ORF8 is a viral immunoglobulin-like (Ig-like) domain protein encoded by the severe acute respiratory syndrome coronavirus 2 (SARS-CoV-2) RNA genome. It tends to evolve rapidly and interfere with immune responses. The full-length SARS-CoV-2 ORF8 is composed of a signal peptide (residues 1-15) and an Ig-like domain (residues 16-121). Herein, we determined the crystal structures of SARS-CoV-2 ORF8 (S84) (one of the epidemic isoforms) and the bat coronavirus RaTG13 ORF8 variant at 1.62 Å and 1.76 Å resolution, respectively.

To determine the sequence-structure relationship, we next solved the crystal structure of the RaTG13 ORF8 Ig-like domain at 1.76 Å, in which the electron density of residues 18-121 can be clearly traced. It is worth noting that there are two molecules in one asymmetric unit, which is different from SARS-CoV-2 ORF8 (S84). Protomers A and B form a dimer via an intermolecular covalent Cys20-Cys20 disulfide bond. Similar to SARS-CoV-2 ORF8, the RaTG13 ORF8 Ig-like domain folds into a “β-sandwich” containing two β-sheets (strands βB, βD, and βE compose the small sheet; strands βA, βC, βC’, βF, and βG compose the large sheet) and an insertion region. However, the insertion region forms a dynamic loop in the RaTG13 ORF8 Ig-like domain, distinguished from the β-hairpin fold in SARS-CoV-2 ORF8 (S84). Unlike SARS-CoV-2 ORF8 (S84), the residues 62-78 loop region of RaTG13 ORF8 is assembled different conformations between the protomer A and protomer B in one asymmetric unit. The electron density of residues 63-65 of RaTG13 ORF8 is unclear, indicating a dynamic region. Additionally, the RaTG13 ORF8 displayed a similar two-stranded parallel β-sheet in protomers A and B’, like SARS-CoV-2 ORF8 (L84). SARS-CoV-2 ORF8 (L84) was the strongest, followed by SARS-CoV-2 ORF8 (S84), and RaTG13 ORF8 was the last.

>SFHQECSLQSCAQHQPYVVDDPCPIHFYSKWYIRVGARKSAPLIELCVDEVGSKSPIQYIDIGNYTVSCSPFTINCQEPKLGSLVVRCSFYEDFLEYHDVRVVLDFI[2x]>MSTNTSKTLELFSKKTVQEHNTANDCWVTYQNRKIYDVTRFLSEHPGGDESILDYAGKDITEIMKDSDVHEHSDSAYEILEDEYLIGYLATDEEAARLLTNKNHKVEVQLSADGTEFDSTTFVKELPAEEKLSIATDYSNDYKKHKFLDLNRPLLMQILRSDFKKDFYVDQIHRPRHYGKGSAPLFGNFLEPLTKTAWWVVPVAWLPVVVYHMGVALKNMNQLFACFLFCVGVFVWTLIEYGLHRFLFHFDDWLPESNIAFATHFLLHGCHHYLPMDKYRLVMPPTLFVILCAPFYKLVFALLPLYWAYAGFAGGLFGYVCYDECHFFLHHSKLPPFMRKLKKYHLEHHYKNYQLGFGVTSWFWDE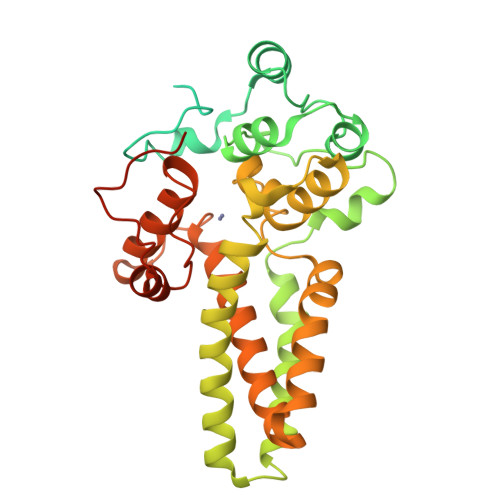VFGTYLGPDAPLSKMKYESGLEVLFQ[2x]Nicotinic acetylcholine receptors (nAChRs) belong to the superfamily of pentameric ligand gated ion channels that are widely expressed in the neuromuscular junction (muscle type), in the central and peripheral neurons as well as in other tissues (neuronal types), and are naturally activated by the neurotransmitter acetylcholine (ACh). The ACh binding site, usually referred to as an orthosteric binding site, is located at the interface between the ECDs of two adjacent subunits, one contributing the principal or (+) side (consisting of loops A, B and C) and the other one contributing the complementary or (−) side (consisting of loops D, E and F). The β3 subunit of nicotinic acetylcholine receptors (nAChRs) participates in heteropentameric assemblies with some α and other β neuronal subunits forming a plethora of various subtypes, differing in their electrophysiological and pharmacological properties. While β3 has for several years been considered an accessory subunit without direct participation in the formation of functional binding sites, recent electrophysiology data have disputed this notion and indicated the presence of a functional (+) side on the extracellular domain (ECD) of β3.

The human β3 ECD was expressed in the yeast Pichia pastoris and after enzymatic deglycosylation, the obtained crystals yielded a 2.4 Å resolution structure of its monomeric state. As shown, the structure of β3 ECD adopts overall the same structural architecture that has been presented previously for homologous proteins. Its main secondary structure elements comprise the N-terminal α-helix and a ten-stranded β-sandwich core, from which several putatively functionally important loops (loops A–F) emerge. Two N-acetylglucosamine (GlcNAC) residues were clearly detected in the electron density maps, modifying predicted glycosylated asparagine residues, one at a highly conserved glycosylation site located at the C-terminal side of the Cys-loop and another at loop β5–β6. On the contrary, loop C was found to be the most diverging region both in terms of sequence and structure with regard to the other nAChR subunits. However, as the crystal structure of β3 ECD shows, another arginine, originating this time from loop C, β3-Arg190, not present in β2 and β4, nor in α subunits, spatially places its guanidine group approximately at the same position as the guanidine group of the β2-Arg149. This in turn induces breakage of the already deficient aromatic box, slightly reorientating the rotamer of loop A Phe94 to create a distorted sandwich cation–pi assembly with Tyr196 for the guanidine group of Arg190. As Arg190 resides in the post β9-strand region, loop C adopts a previously unobserved trajectory with its lower and upper parts obtaining a closed-like conformation and its middle part (tip of loop C) being in an intermediate conformation (closed-in compared to β2 and more open compared to the agonist-bound α4 subunit).

> DYKDDDDKIAENEDALLRHLFQGYQKWVRPVLHSNDTIKVYFGLKISQLVDVDEKNQLMTTNVWLKQEWTDHKLRWNPDDYGGIHSIKVPSESLWLPDIVLFENADGRFEGSLMTKVIVKSNGTVVWTPPASYKSSCTMDVTYFPFDRQNCSMKFGSWTYDGTMVDLILINENVDRKDFFDNGEWEILNAKGMKGNRRDGVYSYPFITYSFVLRRHHHHHH>[4x]PEIITPIITPFTKDNRIDKEKLKIHAENLIRKGIDKLFVNGTTGLGPSLSPEEKLENLKAVYDVTNKIIFQVGGLNLDDAIRLAKLSKDFDIVGIASYAPYYYPRMSEKHLVKYFKTLCEVSPHPVYLYNVPTATGKDIDAKVAKEIGCFTGVKDCIENI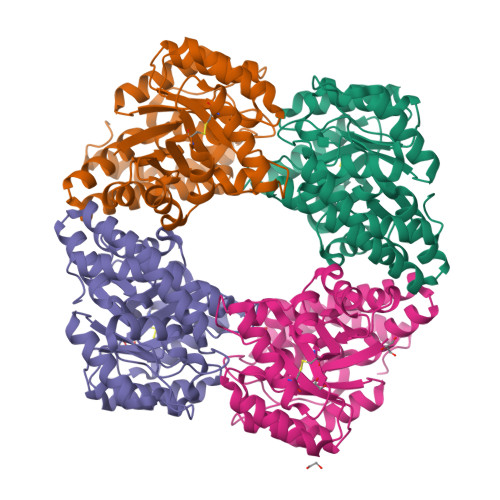IHTLDYKRLNPNMLVYSGSDMLIATVASTGLDGNVAAGSNYLPEVTVTIKKLAMERKIDEALKLQFLHDEVIEASRIFGSLSSNYVLTKYFQGYDLGYPRPPIFPLDDEEERQLIKKVEGIRAKLVELKILKE A trait of BP bacteria is a conserved gene cluster coding for the biosynthesis of polyketides (malleicyprols) with a reactive cyclopropanol unit that is critical for virulence. We show that BurG, an unusual NAD+-dependent member of the ketol-acid reductoisomerase family, constructs the strained cyclopropanol ring. A sequence similarity search using BLAST predicted that BurG belongs to the family of ketol-acid reductoisomerases (KARIs; EC 1.1.1.86), well-characterized enzymes that play key roles in the biosynthesis of branched-chain amino acids. Biochemical assays and a suite of eight crystal structures of native and mutated BurG with bound analogues and inhibitors provide snapshots of each step of the complex reaction mechanism, involving a concealed oxidoreduction and a C–S bond cleavage.

To gain more insight into the reaction mechanism and the role and position of NAD+ in the enzyme, we performed protein crystallography. We raised crystals of holo-BurG in the absence or presence of 7 as surrogate and solved the structures at a resolution of 1.8 Å and 1.9 Å, respectively. Indeed, HR-LCMS analysis of a denatured BurG preparation revealed the presence of the nucleotide cofactor NAD+. The amino acid residues Asn48 and Asp51 exclude the negatively charged phosphate group of NADP+ from binding in the active centre of BurG. A co-crystallized glycerol molecule (used as cryoprotectant) maps the entire specificity pocket next to the catalytic centre. The positioning of NAD+ in the active site of BurG indicates that an oxidation event occurs during cyclopropanol formation. The head region (C1–C3) of all co-crystallized ligands was consistently found to be firmly locked in a conserved binding mode that is facilitated by interactions with the two Mg2+ ions of the enzyme (e for unliganded holo structure).

>MNDLIYQDEHASLQPLEGRTVAVIGYGIQGRAFAANLRDSGVAVRVGNIDDRYFELARAEGHRVTNIAEAVAHADIVLLLIPDEAHGAVFDVDIAPNLRDGALLCVAHGHSLVQGDVRPLPGRDLAMLAPRMYGDPIRRYYLAGQGAPAYFDIVADHTGRARDRVLAIARAVGFTRAGVMALGYRQETFLDLFQEQFLAPALVDLVETGFQVLVERGFNPKAALLEVYGSGEMGKMMLDGADIGLDEVVALQGSPTCQVGYHRWRGRTLPTAVRELAARVLDQIEGGDFSAYLKEQASNDYASLDDARRAALKRPLNVAHAQVRAAFRFPTEAAGGLYQAAQAPADVEPEAAR[2x]> GSHMDDDLVDAEGNLVENGGTYYLLPHIWAHGGGIETAKTGNEPCPLTVVRSPNEVSKGEPIRISSQYRSLFIPRGSLVALGFANPPSCAASPWWTVVDSPQGPAVKLSQQKLPE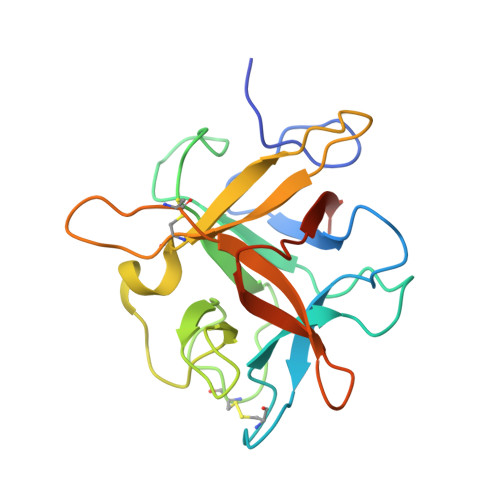KDILVFKFEKVSHSNIHVYKLLYCQHDEEDVKCDQYIGIHRDRNGNRRLVVTEENPLELVLLKAKSETASSH> GPHMPPNRRTCVFFEAPGVRGSTKTLGELLDTGTELPRAIRCLYSRCCFGIWNLTQDRAQVEMQGCRDSDEPGCESLHCDPSPRAHPSPGSTLFTCSCG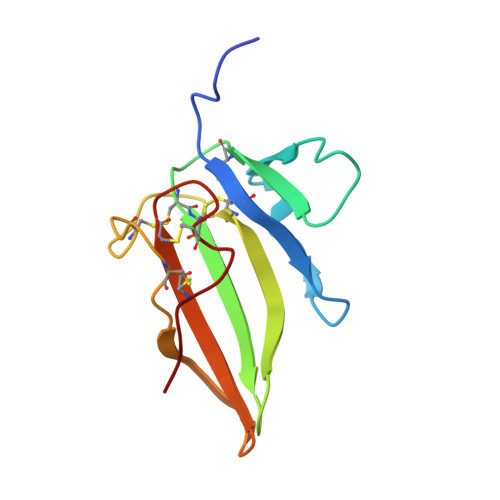TDFCNANYSHLP> HKCDITLQEIIKDLNSLTEQKTLCTELTVTDIFAASKNTTEKETFCRAATVLRQFYSHHEKDTRCLGATAQQFHRHKQLIRFLKRLDRNLWGLAGLNSCPVKEANQSTLENFLERLKTIMREKYSKCSS

Interleukin 4 (IL-4) is a pleiotropic cytokine that plays a major regulatory role in the immune system. Signal transduction of IL-4 is mediated by a sequential binding process, initiated first by binding of IL-4 to its high-affinity single membrane spanning receptor chain IL-4Rα. This intermediate ligand receptor complex then recruits one of two possible low-affinity receptor subunits, the common gamma chain (γc) or the IL-13Rα1 chain, into the functional hetero-trimeric complex to initiate signalling. The overall structure of IL-4 comprises the known four-helical bundle in up-up-down-down topology, which like the crystal packing is unaffected by these mutations.

Analysis of the variants T13D and F82D yielded dissociation constants KD of 0.02 – 0.04 nM and 0.03 – 0.04 nM respectively. The increase in affinity is mainly attributable to the reduced dissociation rates (koff) of T13D and F82D. The structures of the IL-4 variants T13D (max. resolution 1.65 Å), F82D (max. resolution 1.7Å) and T13D-F82D (max. resolution 1.8Å) were refined on the basis of the structure of wild-type IL-4 (max. resolution 1.8Å); all crystals were obtained under identical conditions, allowing detailed comparison. In the variant T13D, the aspartate residue resides in the middle of the first α-helix αA, and the side chain is oriented towards α-helix C. Both carboxylate oxygens of Asp13 are involved in a bi-dentate salt bridge to Arg85 on helix αc, thereby tightly fixing the side chain of Arg85. The geometries and distances of the bi-dentate hydrogen bonds are close to ideal parameters; the planes formed by the carboxylate of Asp13 and the guanidinium group of Arg85 are out of planarity by just 14°; the lengths of the two hydrogen bonds are 2.7 and 2.8Å. The χ1 torsion angle of Arg85 is in the trans conformation (174° IL-4, 176° IL-4 T13D) for both proteins; in the case of IL-4, χ2 of Arg85 is slightly off trans (160°), whereas for T13D, the torsion angle χ2 of Arg85 is in the trans conformation (176°). In contrast, the χ3 torsion angle differs by 115° between IL-4 (58°, gauche- conformation) and T13D (-57°, gauche+ conformation). Modelling of the interaction of T13D bound to IL-4Rα suggests that the guanidinium group of Arg85 (T13D) now forms bi-dentate hydrogen bonds with the main chain carbonyl of the receptor Asp125. In contrast to the hydrogen-bonding network of Arg85 in wild-type IL-4, Arg85 in the complex of T13D:IL-4Rα is probably also fixed to Asp13 (T13D) via a bi-dentate salt bridge. This internal hydrogen bonding would result in fixation of the Arg85 side chain prior to complex formation.>[2x]XSLSDKDKAAVRALWSKIGKSADAIGNDALSRMIVVYPQTKTYFSHWPDVTPGSPHIKAHGKKVMGGIALAVSK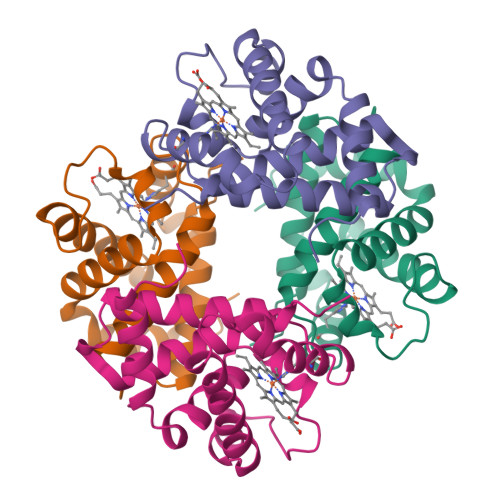IDDLKTGLMELSEQHAYKLRVDPANFKILNHCILVVISTMFPKEFTPEAHVSLDKFLSGVALALAERYR;>[2x]VEWTDKERSIISDIFSHMDYDDIGPKALSRCLIVYPWTQRHFSGFGNLYNAEAIIGNANVAAHGIKVLHGLDRGVKNMDNIAATYADLSTLHSEKLHVDPDNFKLLSDCITIVLAAKMGHAFTAETQGAFQKFLAVVVSALGKQYH> PM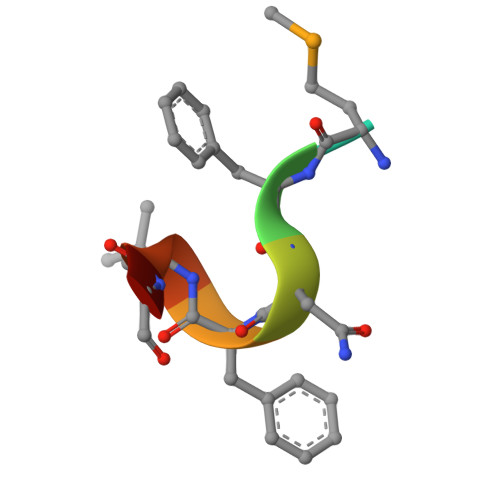FNFLGC> MNTFFLTPAAAAARRVAVSFFARSSASGFPQHRVALRPFPSQRPAERAHNLAKSQTLRSVKAHGRQSGKKEQSTESGGR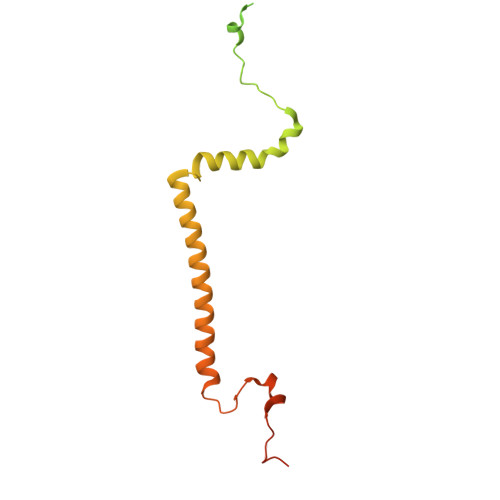RGFRAAVGAGTGCMLAASPMLFTDYDNTASPKSELIFMAGNALGYCTERFFENEYGQSIFMFALGLAYLAMLGHEGKIHGAVWRMKHLFATNFKMVGHPRYAYALPKNPLLQDAAPTKTGSTSAKK Bacillus sp. AHU2216 α-glucosidase (BspAG13_31A), belonging to the glycoside hydrolase family 13 subfamily 31, specifically cleaves α-(1→4)-glucosidic linkages and shows high disaccharide specificity. BspAG13_31A has three domains common to GH13 enzymes: domain A, a catalytic domain that adopts a (β/α)8-barrel fold; domain B, a long loop connecting the third β-strand and third α-helix of domain A (β→α loop 3); domain C, a domain formed by two antiparallel β-sheets that follows domain A. The maltose moiety of G3 and maltotetraose (G4), covering subsites +1 and +2 of this enzyme, adopts a less stable conformation than the global minimum energy conformation, presumably because of steric hindrance by Asn258 at subsite +2. We solved the crystal structures of inactive double mutants, E256Q/N258G and E256Q/N258P, in which the general acid/base catalyst Glu256 was substituted with Gln together with the mutation at Asn258, in complex with G3.

Crystals of E256Q/N258G and E256Q/N258P were prepared by co-crystallization in the presence of 5 mM G3 and G4, respectively, and the structures of E256Q/N258G and E256Q/N258P were solved at 1.7 Å and 1.5 Å resolutions, respectively. Structural analysis of E256Q/N258G and E256Q/N258P in complex with G3 revealed that the conformation of the maltose moiety bound at subsites +1 and +2 of the double-mutant enzymes was different from that of E256Q. Torsion angles of d-glucosyl residues in subsites +1 and +2 of E256Q/N258G and E256Q/N258P were close to the torsion angles of d-glucosyl residues in the stable α-glucan: Φ (5-O, 1-C, 4′-O, 4′C) = 102° and Ψ (1-C, 4′O, 4′-C, 5′-C) = –120°, which is considered the global minimum energy structure. A molecular mechanics study of maltose suggested that torsion angles of d-glucosyl residues at subsite +1 and +2 in the E256Q-G3 complex are less stable than the global minimum, and the conformation of G3 observed in E256Q/N258G and E256Q/N258P is predicted to be more thermodynamically stable than that in E256Q. This conformational difference of G3 presumably arises from the elimination of steric hindrance by Asn258. In the E256Q/N258G-G3 complex, an additional hydrogen bond between Met229 and 3-O of the d-glucose residue at subsite +2 is predicted. This hydrogen bond may stabilize the Michaelis complex and stabilize the transition state because the Km of N258G was 25-fold lower for G3 when compared with that of the wild type. The side chain of Phe282 of E256Q/N258G and E256Q was suitably positioned to interact with the d-glucosyl residue at subsite +2, whereas that of Phe282 in E256Q/N258P was distal from the corresponding d-glucosyl residue and unlikely to have any contact with the substrate. In addition, the carbonyl oxygen of Phe282 was suitably positioned to form a water-mediated hydrogen bond with the d-glucose residue at subsite +2 in E256Q/N258G and E256Q but not in E256Q/N258P.

> MEKKWWKEAVAYQIYPRSFMDSNGDGIGDIQGVISKLDYLSDLGIDVIWICPIYQSPNDDNGYDISDYKDIMKDFGTMEDFDELLDEVHHRGMKLIMDLVINHTSDEHPWFLESRSAKENPYRDYYIWHEGKDGKEPNNWESIFSGSAWEFDEKTKEYYMHVFSKKQPDLNWENEKVRHELYEMVNWWLDKGIDGFRVDAISHIKKVAGFPDLPNPEKLDYVPSFEGHMNRPGIQEHLKELKEKTFAKYDIMTVGQAGGVTSDSADEWVAEDGGNFNMIFQFEHMGLWDKGEEKPLDLIELKTILTNWQNGLEKINGWNALYLENHDQIRSVNKFGSTAYRVESAKCLAALYFLMKGTPFIYQGQELGMTNVKFDSIDDYDDVGMINYYRIQREKGDSHDEIMKVIWETGRDNSRTPMQWNTEKNAGFSTGNPWMKVNPNYVDINVEEQKSDKNSVLNFYKQLIKIRKQHDVLVYGTYKLLAEEDSAIYAYTRTLEGKTAVVICNMSPNNQTFEFPSESSFTNIEVLIHNYPLDKNETLEQCTLHPYETRVYLLSLEHHHHHH> FEFPEELKTKLQEHINYFPKKRQAILLCLHEIQNYYGYIPPESLKPLADMLELPLNHVEGVVAFYDMFDREDKAKYRIRVCVSIVCHLMGTNKLLKALENILGIKPGEVTPDGK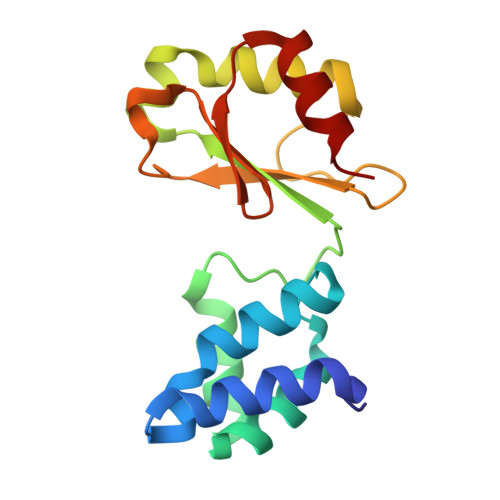FKIVPVQCLGACSEAPVFMVNDDEYKFESEVQLNEILSRYT> GSHMEVLKNIRIYPLSNFITSTKNYINLPNELRNLISEEQESKLGFLHIIESDFKPSVALQKLVNCTTGDEKILIIDIVSIWSQQKQRQHGAIYMNSLSCINITGLIVFLELLYDSPMDALRRCQVDNFNFQLRGIVIDNLSFLNFESDKNYDVINLSKFEKLFKILRKLREFLGCWIITKSFPTDFYNGIENTLVDKWSIKRKSGVTLYPT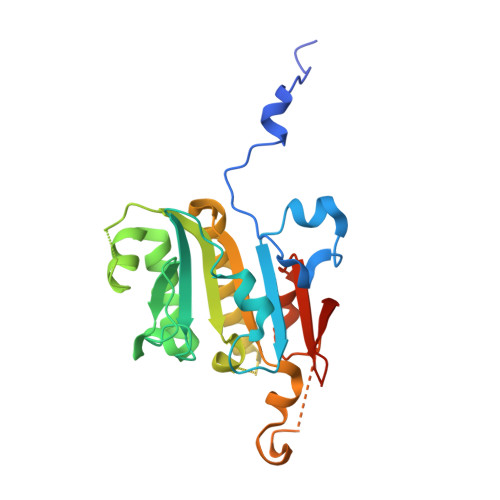KLPDSYMKGMDLIIYREVVDGRPQYRRIAALEE>MDYKDDDDKMQPDMSLNVIKMKSSDFLESAELDSGGFGKVSLAFHRTQGLMIMKTVYKGPNCIEHNEALLEEAKMMNRLRHSRVVKLLGVIIEEGKYSLVMEYMEKGNLMHVLKAEMSTPLSVKGRIILEIIEGMAYLHGKGVIHKDLKPENILVDNDFHIKIADLGLASFKMWSKLNNEEHNELREVDGTAKKNGGTLYYMAPEHLNDVNAKPTEKSDVYSFAVVLWAIFANKEPYENAIAEQQLIMAIKSGNRPDVDDITEYCPREIISLMKLCWEANPEARPTFPGIE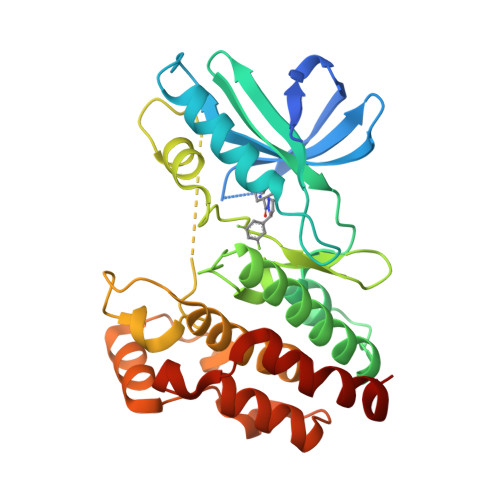EKFRPFYLSQLE[2x]>[2x]MNSTENKNFVISISTAEQRRNHIIEQFTHQNIPFEFFDAFTPSDKLTDHLQRYLPNVANAAQLTMGEKGCLMSHFMLWKKCIDENLDYITLFEDDILLGENANKFLAEGDWLKVRFNFQEIFVLRLETFLMPVQLEKQTQIPPFQQRDIDILTSKHFGTAGYVISQGAAKYLIALFEKLTTEEIKPIDEIMFNQQINATDYRVY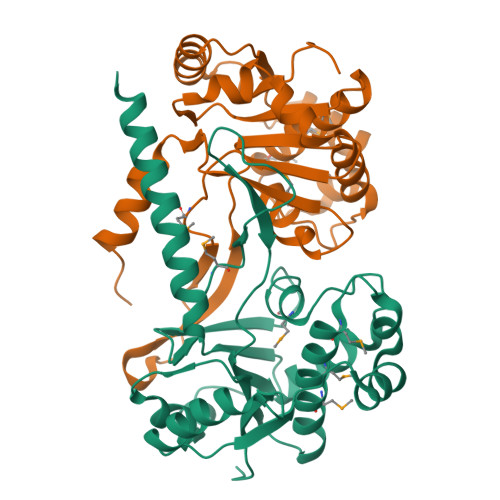QLNPAICVQELQLNQEASLLVSNLEQERKINLKYEKRKHLEHHHHHH> PAKKPYNKIVSHLLVAEPEKIYAMPDPTVPDSDIKALTTLCDLADRELVVIIGWAKHIPGFSTLSLADQMSLLQSAWMEILILGVVY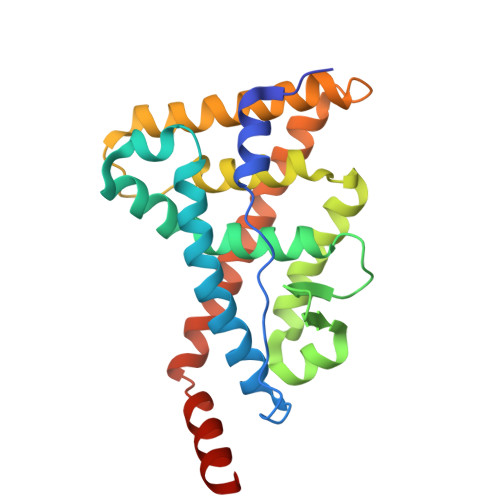RSLSFEDELVYADDYIMDEDQSKLAGLLDLNNAILQLVKKYKSMKLEKEEFVTLKAIALANSDSMHIEDVEAVQKLQDVLHEALQDYEAGQHMEDPRRAGKMLMTLPLLRQTSTKAVQHFYNIKLEGKVPMHKLFLEMLEAKV>[12x]ALESAQESHALHHQNAAALRFQFHITREQAREIVKLCPNCPDWGHAPQLGVNPRGLKPRVLWQMDVTHVSEFGKLKYVHVTVDTYSHFTFATART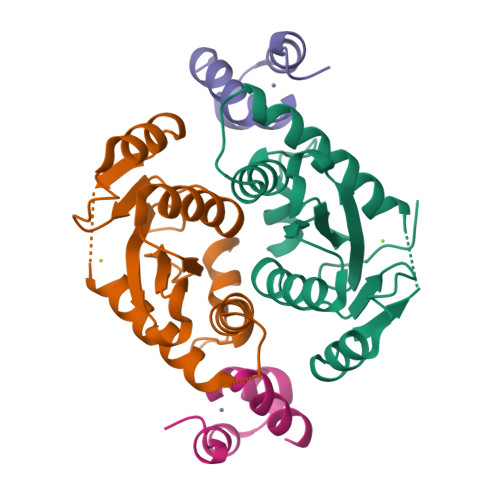GEATKDVLQHLAQSFAYMGIPQKIKTDNAPAYVSRSIQEFLARWKISHVTGIPYNPQGQAIVERTHQNIKAQLNKLQKAGKYYTPHHLLAHALFVLNHVNMDNQGHTAAERHWGP>MKMPAYEFWFVVGSQHLYGDEALAQVEAHAREMVPALQAAVGNAHVLRWKGVLKDADEIRRLCLEASADDVCAGVIAWMHTFSPAKMWIRGLLALRKPLLHLHTQFNRDIPWDTIDMDFMNLNQSAHGDREYGFIGARMGVARKVVVGHWEDPEVRERLAKWMRTAVAFAESRNLKVARFGDNMREVAVTEGDKVGAQIQFGWSVNGYGIGDLVQYIRDVSEQKVNELLDEYEELYDIVPAGRQEGPVRESIREQARIELGLKAFLQDGNFTAFTTTFEDLHGLKQLPGLAVQRLMQQGYGFAGEGDWKTAALLRIMKVMSTGLQGGTSFMEDYTYHFEKGNDLVLGSHMLEVCPSIAAEEKPILDVQHLGIGGKDDPARLVFDGGEGAAVNASLIDLGHRFRLIVNEVDAVKPEHDMPK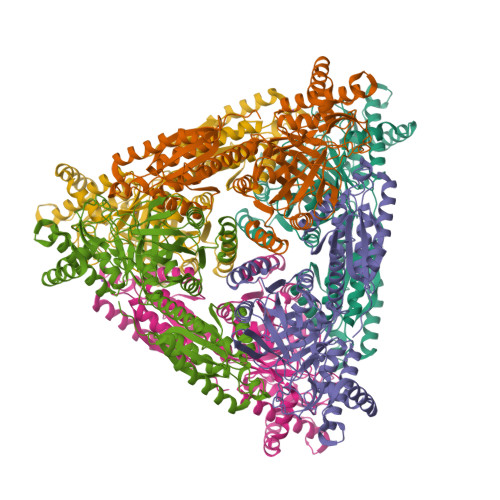LPVARILWKPRPSLRDSAEAWILAGGAHHTCFSFAVTTEQLQDFAEMAGIECVVINEHTSVSSFKNELKWNEVFWRGR[12x]> REFTIDFSTQQSYVSSLNSIRTEISTPLEHISQGTTSVSVINHTPPGSYFAVDIRGLDVYQARFDHLRLIIEQNNLYVAGFVNTATNTFYRFSDFTHISVPGVTTVSMTTDSSYTTLQRVAALERSGMQISRHSLVSSY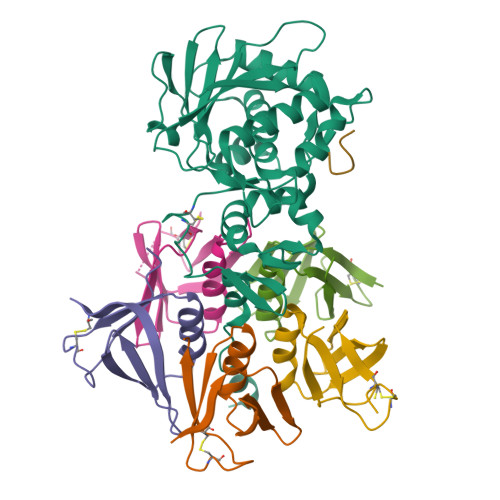LALMEFSGNTMTRDASRAVLRFVTVTAEALRFRQIQREFRQALSETAPVYTMTPGDVDLTLNWGRISNVLPEYRGEDGVRVGRISFNNISAILGTVAVILNCHHQGARSVRAVNEDSQPECQITGDRPVIKINNTLWESNTAAAFLNRKSQFLYTTGK;>[5x]ADCAKGKIEFSKYNEDDTFTVKVDGKEYWTSRWNLQPLLQSAQLTGMTVTIKSSTCESGSGFAEVQFNND;> GFGLFD>ETGKHNCFCIQEVVSGLRQPVGALHSGDGSQRLFILEKEGYVKILTPEGEIFKEPYLDIHKLVQSGIKGGDERGLLSLAFHPNYKKNGKLYVSYTTNQERWAIGPHDHILRVVEYTVSRKNPHQVDLRTARVFLEVAELHRKHLGGQLLFGPDGFLYIILGDGMITLDDMEEMDGLSDFTGSVLRLDVDTDMCNVPYSIPRSNPHFNSTNQPPEVFAHGLHDPGRCAVDRHPTDININLTILCSDSNGKNRSSARILQIIKGKDYESEPSLLEFKPFSNGPLVGGFVYRGCQSERLYGSYVFGDRNGNFLTLQQSPVTKQWQEKPLCLGTSGSCRGYFSGHILGFGEDELGEVYILSSSKSMTQTHNGKLYKIVDPKRPLMPEECRATVQPAQTLTSECSRLCRNGYCTPTGKCCCSPGWEGDFCRTAKCEPACRHGGVCVRPNKCLCKKGYLGPQCEQVDGTKHHHHHH[3x]

Hedgehog-Interacting Protein (HHIP), the only reported secreted inhibitor of Sonic Hedgehog (SHH) signalling, binds directly to SHH with high nanomolar affinity, sequestering SHH. HHIP is composed of an N-terminal domain (HHIP-N) that shows weak sequence homology to the cysteine-rich domain (CRD) superfamily, typically involved in small molecule-binding. The C-terminal domain of HHIP is composed of a β-propeller and two EGF repeats (HHIP-C). Our data suggest a multimodal mechanism, in which HHIP can bind two specific sites on the SHH morphogen, alongside multiple GAG interactions, to inhibit SHH signalling.

To structurally characterise HHIP-C:GAG interactions, we determined the 2.7 Å resolution crystal structure of HHIP-C in complex with a 30-mer heparin molecule. HHIP-C comprises an N-terminal 6-bladed β-propeller and 2 C-terminal EGF repeats, previously identified in the complex of HHIP-C with HhN ligands. The heparin chain contacts two separate clusters of HHIP surface residues (GAG ‘site1’ and GAG ‘site 2’) at either end of the molecule. In this arrangement, a HHIP-C anti-parallel dimer coordinates one single heparin chain by using a central positively-charged region formed by residues from both HHIP protomers. The heparin backbone displays a right-handed helical structure with roughly 4 sugars per turn, in agreement with previous structural studies. A total of 8 monosaccharides are resolved in the structure, running from a reducing (O1; sugar I) to a non-reducing end (O4; sugar VIII) and forming hydrogen bonds with several polar side chains. We also determined the crystal structure of a HHIP-C:SOS complex, which exhibits the equivalent anti-parallel, dimeric HHIP arrangement bound to two SOS molecules coordinated at the same site compared to heparin. In summary, our HHIP-C crystal structures in complex with GAG molecules identify two discrete GAG-binding sites on the surface of HHIP-C, which are distinct and non-overlapping with the HhN-binding interface, thus suggesting that both GAG- and HhN-binding can occur simultaneously. Our HHIP-C:heparin complex structure also suggests that GAGs can mediate the formation of long oligomeric chains of HHIP. We observe two HHIP oligomerisation interfaces - an anti-parallel ‘head-to-tail’ heparin-bound HHIP-C dimer with a total buried surface area of 603 Å2, and a ‘head-to-head’ dimer with a buried surface area of 981 Å2 in the crystal. The ‘head-to-tail’ dimer interface is smaller than physiological dimer interfaces and is likely stabilised by the heparin molecule (PISA ΔiG P-value = 0.41, shape complementarity score = 0.75), while the larger ‘head-to-head’ interface is more likely to be physiological (PISA: ΔiG P-value = 0.43, shape complementarity score: 0.52).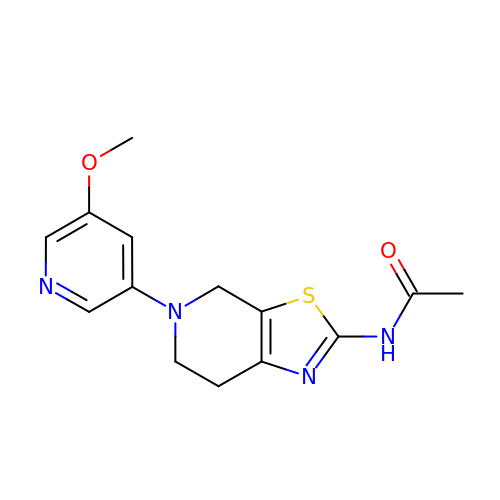N-[5-(5-methoxypyridin-3-yl)-4,5,6,7-tetrahydro[1,3]thiazolo[5,4-c]pyridin-2-yl]acetamide | C14 H16 N4 O2 S | BJLFVHWVPYZOBS-UHFFFAOYSA-N>NEAIECHLSDLLQQLTSVNASKPSERGLVRQEEAEDPACIPIFWVSKWVDYSDKYGLGYQLCDNSVGVLFNDST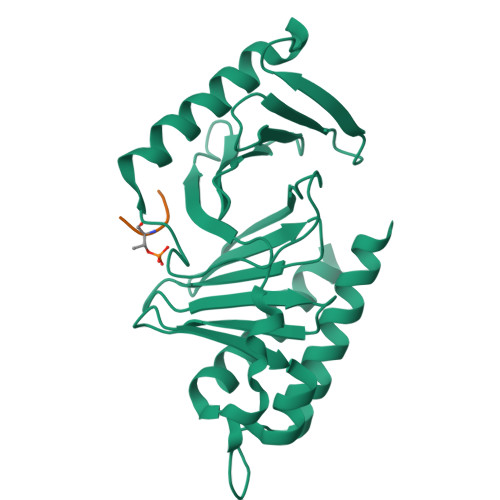RLILYNDGDSLQYIERDGTESYLTVSSHPNSLMKKITLLNYFRNYMSEHLLKAGANITPREGDELARLPYLRTWFRTRSAIILHLSNGTVQINFFQDHTKLILCPLMAAVTYINEKRDFQTYRLSLLEEYGCCKELASRLRYARTMVDKLLSSRSASNRLKAS[2x];>[2x]FSQHKTSTI The P pilus, produced in uropathogenic Escherichia coli, displays the adhesin PapG responsible for targeting the bacterium to the kidney epithelium. The PapA rod is formed by more than 1,000 PapA molecules assembled in a right-handed helical manner, with 3.3 molecules per turn. In a process called donor–strand complementation (DSC), the G1 β-strand of PapD inserts a conserved motif of three alternating hydrophobic residues (called the P1 to P3 residues) plus N101 (P4 residue) into four binding pockets in the hydrophobic groove of the pilus subunits (P1 to P4 binding pockets).

In order to investigate the PapD/PapA and PapA/PapA interactions within the P pilus rod, the first structure which we solved was that of PapD/PapA, where two mutations were introduced in the papA gene. This was necessary because PapA in purified wild-type PapD/PapA complexes tends to spontaneously polymerize, and self-polymerization of PapA has prevented structural studies. Thus, in addition to the G15N mutation, a mutant where residues 2 to 8 were deleted was next constructed. The deleted region is just N-terminal to the DSE region of the Nte of PapA. This mutant (PapANtd1_G15N) did not undergo spontaneous polymerization, and formed a stable complex with PapD. Crystals of PapD/PapANtd1_G15N diffracted to a resolution of 2.6 Å, and the structure was solved by molecular replacement using the PapD/PapK structure as a search model. This structure is very similar to the already known PapD/PapK, PapD/PapENtd, or PapD/PapHNtd1 structures. Like PapK, PapE, or PapH, PapA lacks strand G of its Ig-fold; PapD complements this by donating its G1 strand.

>AVSLDRTRAVFDGSEKSMTLDISNDNKQLPYLAQAWIENENQEKIITGPVIATPPVQRLEPGAKSMVRLSTTPDISKLPQDRESLFYFNLREIPPRSEKANVLQIALQTKIKLFYRPAAIKTRPNEVWQDQLILNKVSGGYRIENPTPYYVTVIGLGGSEKQAEEGEFETVMLSPRSEQTVKSANYNTPYLSYINDYGGRPVLSFICNGSRCSVKKEK[4x];>[4x]APTIPQGQGKVTFNNTVVDAPCSISQKSADQSIDFGQLSKSFLEAGGVSKPMDLDIELVNCDITAFKGGNGAKKGTVKLAFTGPIVNGHSDELDTNGGTGTAIVVQGAGKNVVFDGSEGDANTLKDGENVLHYTAVVKKSSAVGAAVTEGAFSAVANFNLTYQ> GANSNDIHLLKDS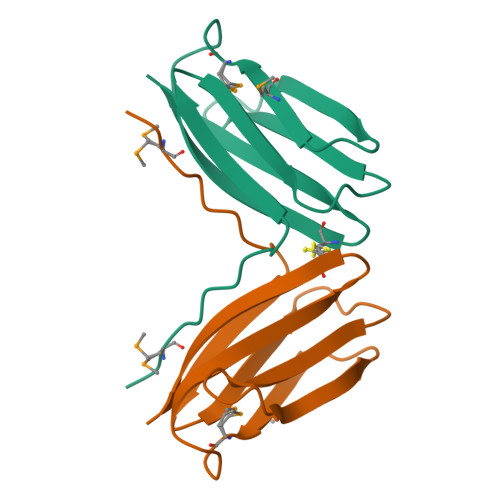RSNPMGIPIQPTYEKCAILSNILNVSFGRAKDYAIITVTNKATGEIVHSKTYHNTSIVMIDMSSCEKGEYTIHIILNDCLLEGTFTVQ>TVSFNPYEPELAP[2x];>[2x]GSLIGLMKDAFQPHHHHHHHLSPHPPGTVDKKMVEKCWKLMDKVVRLCQNPKLALKNSPPYILDLLPDTYQHLRTILSRYEGKMETLGENEYFRVFMENLMKKTKQTISLFKEGKERMYEENSQPRRNLTKLSLIFSHMLAELKGIFPSGLFQGDTFRITKADAAEFWRKAFGEKTIVPWKSFRQALHEVHPISSGLEAMALKSTIDLTCNDYISVFEFDIFTRLFQPWSSLLRNWNSLAVTHPGYMAFLTYDEVKARLQKFIHKPGSYIFRLSCTRLGQWAIGYVTADGNILQTIPHNKPLFQALIDGFREG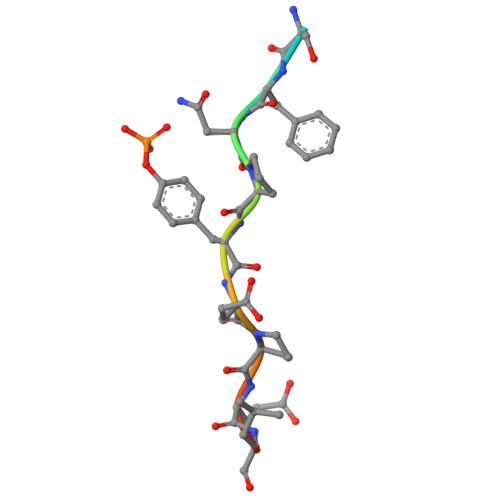FYLFPDGRNQNPDLTG4-{[(1R,3S)-3-amino-2,2,3-trimethylcyclopentyl]amino}-6-phenylpyrrolo[1,2-b]pyridazine-3-carboxamide 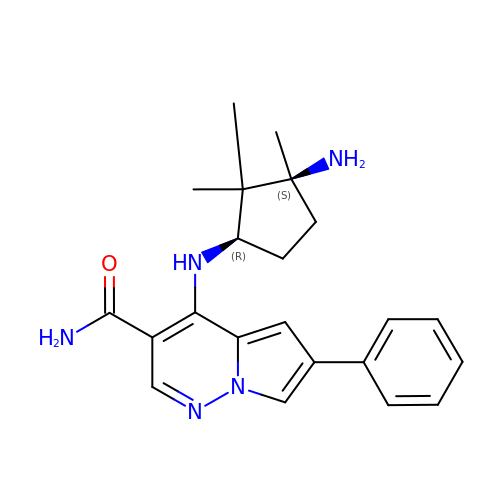| C22 H27 N5 O | DIFGSGNUHRNWPK-GCJKJVERSA-N>TTGHSYEKYNNWETIEAWTKQVTSENPDLISRTAIGTTFLGNNIYLLKVGKPGPNKPAIFMDCGFHAREWISHAFCQWFVREAVLTYGYESHMTEFLNKLDFYVLPVLNIDGYIYTWTKNRMWRKTRSTNAGTTCIGTDPNRNFDAGWCTTGASTDPCDETYCGSAAESEKETKALADFIRNNLSSIKAYLTIHSYSQMILYPYSYDYKLPENNAELNNLAKAAVKELATLYGTKYTYGPGATTIYPAAGGSDDWAYDQGIKYSFTFELRDKGRYGFILPESQIQATCEETMLAIKYVTNYVLGHL[3x];>RKVYAF[3x]

The carboxypeptidase TAFIa (activated thrombin activatable fibrinolysis inhibitor) is a central player in fibrinolysis. TAFIa removes carboxy-terminal lysines and arginines from partially degraded fibrin. Carboxypeptidase B (CPB) was used instead of TAFIa for practical reasons, since TAFIa was found to be highly unstable with a half-life of approximately 2h at 22 °C30. CPB, on the other hand, is stable and highly homologous to TAFIa with 48% sequence identity.

The known anabaenopeptins B, C, and F (1, 2 and 3) were isolated from a culture of the cyanobacterium Planktothrix rubescens and tested for their inhibitory activity against TAFIa in an enzymatic assay. Compounds 1–3 turned out to be potent inhibitors of TAFIa with IC50 values of 1.5, 1.9 and 1.5 nM, respectively. An equivalent order was found for 2, 1 and 13 with IC50 values of 1.9 nM, 1.5 nM and 440 nM for the Lys, Arg and Tyr side chains. In addition, we obtained crystal structures of the complexes of anabaenopeptin B (1), anabaenopeptin C (2) and anabaenopeptin F (3) with the surrogate protease carboxypeptidase B (CPB). We used CPB crystals grown in the presence of ε-caproic acid with space group P32, since these crystals had wide solvent channels, which allowed the soaking-in of large inhibitors like the anabaenopeptins. After soaking, the crystals diffracted to 2.0–2.3 Å, enabling the calculation of detailed and accurate electron density maps. The general binding modes of 1–3 were found to be very similar and in the following discussion the complex with 2 is used as an example. The linear part of the anabaenopeptins, which mimics the carboxy-terminus of the TAFIa substrate fibrin, deeply penetrated the active site channel and bound in the carboxylate- and specificity-pockets, while the circular parts of the anabaenopeptins were positioned in the entrance of the channel and completely blocked the channel like a plug, thereby preventing other molecules from entering it. All hydrogen bond donor and acceptor atoms of 2 interacted either with hydrogen bond donor/acceptors from the protein, or with bound water molecules. We found that the C-terminal arginine or lysine side chain (R1 in Fig. 3) bound in the S1’ binding pocket and interacted with the side chains of Asp255 and Ser207. The R1 residue was bound in the S1’ pocket, which is specific for basic residues like arginine and lysine in TAFIa and CPB, while the S1’ pocket of CPA is specific for large apolar residues like phenylalanine and isoleucine.>[2x]MAQFVYTMHRVGKVVPPKRHILKNISLSFFPGAKIGVLGLNGAGKSTLLRIMAGIDKDIEGEARPQPDIKIGYLPQEPQLNPEHTVRESIEEAVSEVVNALKRLDEVYALYADPDADFDKLAAEQGRLEEIIQAHDGHNLNVQLERAADALRLPDWDAKIANLSGGERRRVALCRLLLEKPDMLLLDEPTNHLDAESVAWLERFLHD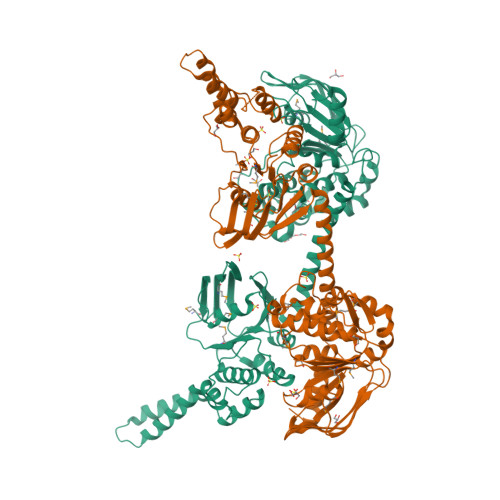FEGTVVAITHDRYFLDNVAGWILELDRGEGIPWEGNYSSWLEQKDQRLAQEASQEAARRKSIEKELEWVRQGTKGRQSKGKARLARFEELNSTEYQKRNETNELFIPPGPRLGDKVLEVSNLRKSYGDRLLIDDLSFSIPKGAIVGIIGPNGAGKSTLFRMISGQEQPDSGTITLGETVKLASVDQFRDSMDNSKTVWEEVSGGLDIMKIGNTEMPSRAYVGRFNFKGVDQGKRVGELSGGERGRLHLAKLLQVGGNMLLLDEPTNDLDIETLRALENALLEFPGCAMVISHDRWFLDRIATHILDYQDEGKVEFFEGNFTEYEEYKKRTLGADALEPKRIKYKRIAK>MAKEKGLTPQSQDFSEWYLEVIQKAELADYGPVRGTIVVRPYGYAIWENIQQVLDRMFKETGHQNAYFPLFIPMSFLRKEAEHVEGFSPELAVVTHAGGEELEEPLAVRPTSETVIGYMWSKWIRSWRDLPQLLNQWGNVVRWEMRTRPFLRTSEFLWQEGHTAHATREEAEEEVRRMLSIYARLAREYAAIPVIEGLKTEKEKFAGAVYTTTIEALMKDGKALQAGTSHYLGENFARAFDIKFQDRDLQVKYVHTTSWGLSWRFIGAIIMTHGDDRGLVLPPRLAPIQVVIVPIYKDESRERVLEAAQGLRQALLAQGLRVHLDDRDQHTPGYKFHEWELKGVPFRVELGPKDLEGGQAVLASRLGGKETLPLAALPEALPGKLDAFHEELYRRALAFREDHTRKVDTYEAFKEAVQEGFALAFHCGDKACERLIQEETTATTRCVPFEAEPEEGFCVRCGRPSA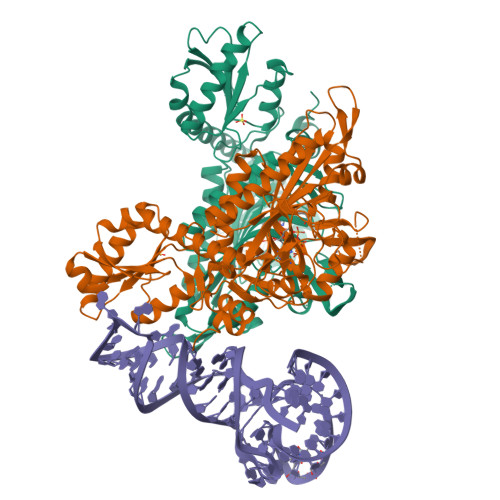YGKRVVFAKAY[2x]>[6x]MSGSHHHHHHSGSMSERPSDLVVNRLVLFVVKGTATATHNTVKPLILLEELGVPHDIYVVEKVSAPWFSEINPHKMVPAILDRSPDGRDTLRAWESTSTLMYIADAYDKDGTFGGRNVQERSEINNWLTLHTAALGPTAKYWLYFYKLHPEKLPKTIEKLRSNITVQYDILERRLNEPGQQYLALKDRPTIADIAT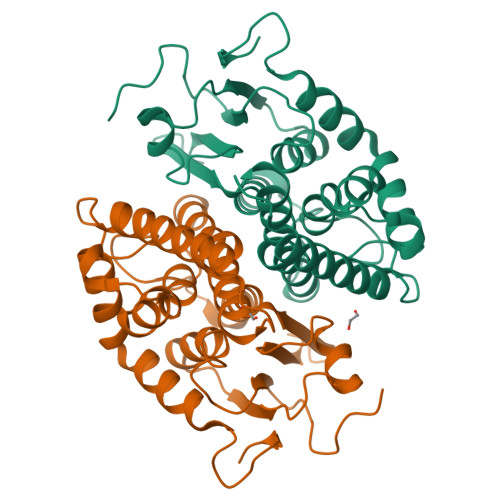LPFAMKSTAELFGLEFEKWPKLQEWSVRMGEREAVKRAWQRVAGFGHGEKEYGMLEA> GPHMSIINYNEGQWSPNNPSG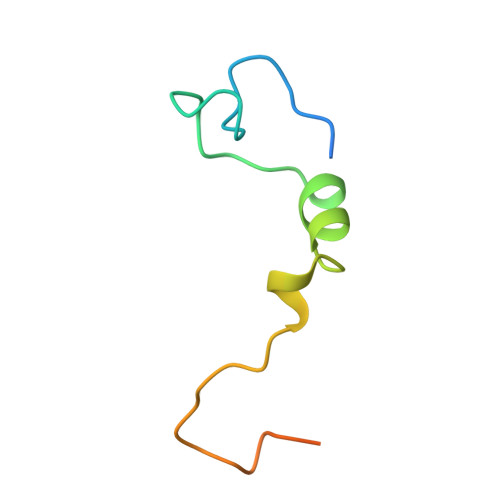KKQYDREQLLQLREVKASRIQPEVKNVSILPQPNLMPSFIRNN>[4x]MIHMRTGVIGVGHLGRFHAQKYAAISQLAGVFDENAE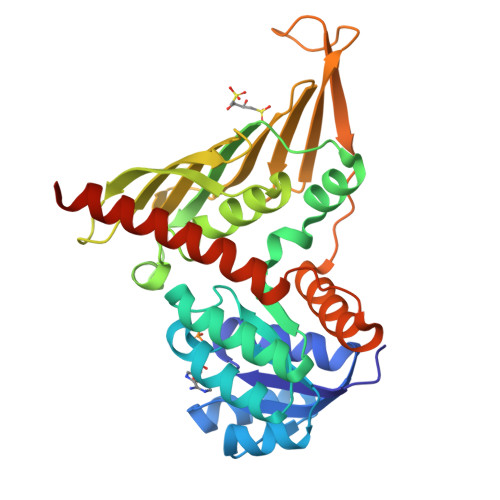RAAEVAAELRCRAFPSVDALLAEVDAVSIVTPTSTHFAVAEVAMQAGVHCLIEKPFTLDTEEADALIGMAQERHLVLAIGHIKRVHPAIQYLRQAGFGAPRYLEAERLAPFKPRSLDIDVIMDLMIHDLDLTLLLTGAEPVDVRAVGVAAVTDKADMATAWMTLNNGTVANLAASRVVREPARRMRIFWQDRYASVDFLNNTLHIYHRGAGTVPGIPGVRDEAVDLAKRDALAAEIEDFLNAIAAHRPVFCDGVAGRRVLAAALQVRVAVEAFLQRLEHHHHHH> SEDSFFSAT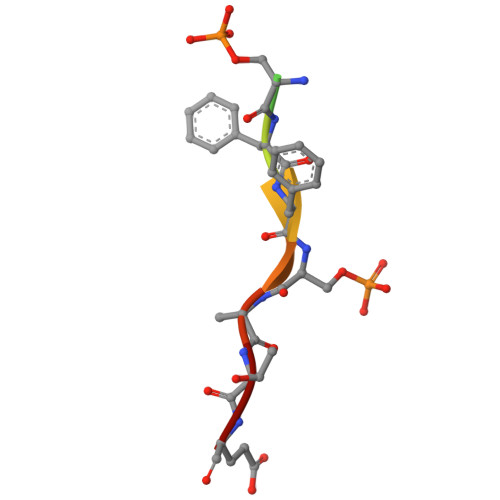E> VKEEIQAKEYLENLNKELAKRTNVETEAAWAYGSNITDENEKKKNEISAELAKFMKEVASDTTKFQWRSYQSEDLKRQFKALTKLGYAALPEDDYAELLDTLSAMESNFAKVKVCDYKDSTKCDLALDPEIEEVISKSRDHEELAYYWREFYDKAGTAVRSQFERYVELNTKAAKLNNFTSGAEAWLDEYEDDTFEQQLEDIFADIRPLYQQIHGYVRFRLRKHYGDAVVSETGPIPMHLLGNMWAQQWSEIADIVSPFPEKPLVDVSAEMEKQGYTPLKMFQMGDDFFTSMNLTKLPQDFWDKSIIEKPTDGRDLVCHASAWDFYLIDDVRIKQCTRVTQDQLFTVHHELGHIQYFLQYQHQPFVYRTGANPGFHEAVGDVLSLSVSTPKHLEKIGLLKDYVRDDEARINQLFLTALDKIVFLPFAFTMDKYRWSLFRGEVDKANWNCAFWKLRDEYSGIEPPVVRSEKDFDAPAKYHISADVEYLRYLVSFIIQFQFYKSACIKAGQYDPDNVELPLDNCDIYGSAAAGAAFHNMLSMGASKPWPDALEAFNGERIMSGKAIAEYFEPLRVWLEAENIKNNVHIGWTTSNKCVS;>VW[2x]

Angiotensin-I-converting enzyme (ACE, EC 3.4.15.1) is a promiscuous zinc metallopeptidase with a number of substrates, including the vasoregulatory peptides angiotensin I and bradykinin, the anti-fibrotic agent N-acetyl-SDKP, the neurotransmitter substance P, and amyloid-β peptide. Here, we present the use of the Drosophila melanogaster ACE homologue, AnCE (which, in particular, shares enzymatic properties with cACE), as a model to study the structural basis of ACE inhibition. The active site is located at the centre of this channel, marked by the location of the catalytic zinc ion, which is coordinated by His367, His371, and Glu395. The high-resolution crystal structures of AnCE in complex with the dipeptides VW, IW, YW, RW, and WR presented here reveal dual binding in both the non-prime (dipeptide-1) and prime (dipeptide-2) subsites of AnCE.

The dipeptides with a C-terminal tryptophan (IW, VW, YW, RW) show an identical conformation of binding within the non-prime subsite, with the tryptophan residue occupying the S2 subsite. IW-1 isoleucine and VW-1 valine sit within the S1 subsite, forming a hydrophobic contact with Trp341. Due to the similarity of isoleucine and valine, the interactions within the S1′ subsite for VW-2 and IW-2 are conserved. Based on this, it is likely that the difference in the dipeptide affinities towards AnCE (IW: 0.08 mM, VW: 0.17 mM) is influenced by the difference in hydrophobicity, with a more hydrophobic side chain being favoured. The tryptophan binding within the S2′ subsite is conserved between IW-2, VW-2, YW-2, and RW-2, where the tryptophan side chain forms hydrophobic interactions with Phe441 and Tyr507, a π-stacking interaction with Phe511, and a H-bond with Gln266. The VW dipeptide has a slightly lower affinity for AnCE, with a Ki value of 117 µM; interestingly, VW also has a lower affinity for cACE when compared to IW, with a Ki value of 2.1 µM. Though VW has lower affinity for cACE and AnCE than IW, it shows higher selectivity when the affinities are compared to nACE, with VW having a Ki value of 151.6 µM compared to IW having a Ki value of 59.6 µM. The difference in affinity between IW and VW in AnCE is likely due to the extra carbon atom in isoleucine, which has an effect on the van der Waals interactions within both subsites, potentially further stabilising the dipeptide compared to VW. The changes within the S1 subsite could influence the more hydrophobic dipeptides IW-1 and VW-1, particularly due to the S1 subsite environment being less favourable for the isoleucine and valine. The S1′ and S2′ subsite changes between AnCE and cACE could result in higher affinity binding of the IW-2 and VW-2 dipeptides within these subsites due to the changes from AnCE-Thr364 and Gln266 to cACE-Val380 and Thr282, respectively, resulting in more hydrophobic pockets.>GIDPFTVPLIFKIGYNVIPLQDVILPTPSSKVLKYLIQSGKLLPSLNNLITSRDKYKPIFISHLGLNQRRIFQTNGNLKTISRGSKLSSTIAFSTQVNVLPELDEGVFETIYGKFHITIESVEIVEVEKLKEEVEKHMNDNIRVRFISPTLLSSKVLLPPSLSERYKRVNAGYSTLPSVGLIVAYAYNVYCNLIGKKEVEVRAFKFGVISNALSRIIGYDLHPVTIVIGEDSKGNLRKARGVMGWIEFDIPDEKLKRRALRYLLASSYLGIGRSRGIGFGEIKLEFIKREENH[4x]

In type I and III systems, pre-crRNA is processed by the Cas6 endonuclease, whereas type II systems utilize an alternative method involving host RNase III. Cas6 proteins typically consist of two tandem RRM (RNA-recognition motif)-like folds {also known as RAMP (repeat-associated mysterious protein) domains } with a diagnostic glycine-rich loop near the C-terminus. In the present paper, we report the crystal structure and accompanying biochemical data for Cas6 from the crenarchaeon Sulfolobus solfataricus. The crystal structure of S. solfataricus Cas6 has revealed a dimeric organization that may be relevant for its in vivo function as a stand-alone crRNA-processing endonuclease.

Although native SsoCas6 crystallized readily, reductive methylation of the surface lysine residues was required to produce well-diffracting crystals. A selenomethionine derivative of the methylated protein was used to solve the structure with a SAD dataset collected to 2.8 Å (1 Å=0.1 nm) resolution. Residues 43–50 and 90–93 are disordered in each of the four monomers in the crystallographic asymmetric unit. The monomer consists of eleven β-strands and eight helices arranged as two tandem RAMP folds linked by a single helix, consistent with the canonical Cas6 fold. The N-terminal RAMP domain of SsoCas6 deviates from the standard motif in that the second RAMP helix (α2) that normally precedes β4 is missing and replaced by a loop with an extended conformation. In the C-terminal RAMP domain, there are three additional helices located on the helical face of the domain as well as a β-hairpin that connects two strands of the central β-sheet. Analysis with the PDBePISA server indicates that the four SsoCas6 monomers in the asymmetric unit assemble into two identical dimers (complexation significance score of 1), consistent with gel-filtration data that also suggested a dimer. The dimer interface was formed between the C-terminal domains of both proteins with an average buried surface area of 1349 Å2. The three non-conserved helices of the C-terminal domain are positioned at the interface and may be responsible for causing dimerization in a Cas6 protein that is typically monomeric. In fact, there were no histidine residues located around the putative active site.>TADELVFFVNGKKVVEKNADPETTLLAYLRRKLGLRGTKLGCGEGGCGACTVMLSKYDRLQDKIIHFSANACLAPICTLHHVAVTTVEGIGSTKTRLHPVQERIAKSHGSQCGFCTPGIVMSMYTLLRNQPEPTVEEIEDAFQGNLCRCTGYRPILQGFRTFAK[2x];>PKQLRFEGERVTWIQASTLKELLDLKAQHPEAKLVVGNTEIGIEMKFKNQLFPMIICPAWIPELNAVEHGPEGISFGAACALSSVEKTLLEAVAKLPTQKTEVFRGVLEQLRWFAGKQVKSVASLGGNIITASPISDLNPVFMASGTKLTIVSRGTRRTVPMDHTFFPSYRKTLLGPEEILLSIEIPYSREDEFFSAFKQASRREDDIAKVTCGMRVLFQPGSMQVKELALCYGGMADRTISALKTTQKQLSKFWNEKLLQDVCAGLAEELSLSPDAPGGMIEFRRTLTLSFFFKFYLT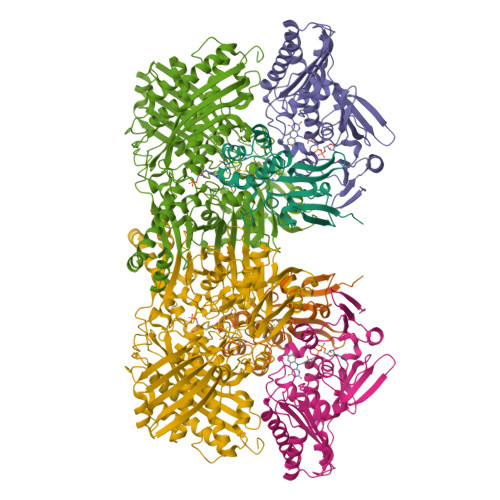VLKKLG[2x];>[2x]DTVGRPLPHLAAAMQASGEAVYCDDIPRYENELFLRLVTSTRAHAKIKSIDVSEAQKVPGFVCFLSADDIPGSNETGLFNDETVFAKDTVTCVGHIIGAVVADTPEHAERAAHVVKVTYEDLPAIITIEDAIKNNSFYGSELKIEKGDLKKGFSEADNVVSGELYIGGQDHFYLETHCTIAIPKGEEGEMELFVSTQNAMKTQSFVAKMLGVPVNRILVRVKRMGGGFGGKETRSTLVSVAVALAAYKTGHPVRCMLDRNEDMLITGGRHPFLARYKVGFMKTGTIVALEVDHYSNAGNSRDLSHSIMERALFHMDNCYKIPNIRGTGRLCKTNLSSNTAFRGFGGPQALFIAENWMSEVAVTCGLPAEEVRWKNMYKEGDLTHFNQRLEGFSVPRCWDECLKSSQYYARKSEVDKFNKENCWKKRGLCIIPTKFGISFTVPFLNQAGALIHVYTDGSVLVSHGGTEMGQGLHTKMVQVASKALKIPISKIYISETSTNTVPNSSPTAASVSTDIYGQAVYEACQTILKRLEPFKKKNPDGSWEDWVMAAYQDRVSLSTTGFYRTPNLGYSFETNSGNAFHYFTYGVACSEVEIDCLTGDHKNLRTDIVMDVGSSLNPAIDIGQVEGAFVQGLGLFTLEELHYSPEGSLHTRGPSTYKIPAFGSIPTEFRVSLLRDCPNKKAIYASKAVGEPPLFLGASVFFAIKDAIRAARAQHTNNNTKELFRLDSPATPEKIRNACVDKFTT> GV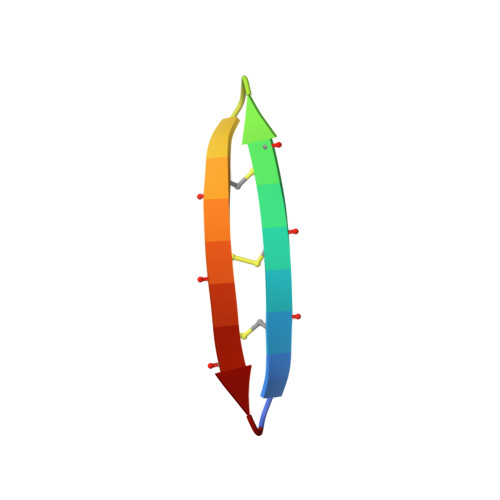CRCVCRRGVCRCVCRR>MRKIRNLLLTLYFYFIATVYIVFYGGFVLFRSFLMRDREKARKYVLKEIEKFGKRAFTWLFSDVVVEGSENIPKDRNFIVVANHQSLMDIPLILGFVATGAFIAKEELRKIPGVNWYIRYLNGVFLDRKNPRRAVRALREAIEKLKNGVTFIVFPE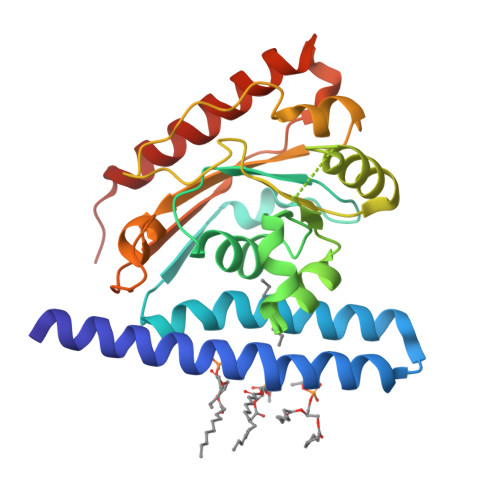GTRSPDGKVLSFKKDSLMIAVKTGVPVLPVSIWGTYHLIPKGRWTFTPGKVFLKIHEPVDPKGFSSEEELRKYVEEVVKRGVEELKARWSK[2x]> MPQHDQLHRYLFENFAVRGELVTVSETLQQILENHDYPQPVKNVLAELLVATSLLTATLKFDGDITVQLQGDGPMNLAVINGNNNQQMRGVARVQGEIPENADLKTLVGNGYVVITITPSEGERYQGVVGLEGDTLAADLEDYFMRSEQLPTRLFIRTGDVDGKPAAGG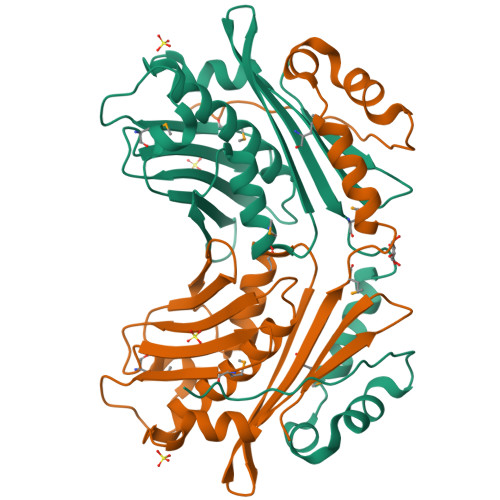MLLQVMPAQNAQQDDFDHLATLTETIKTEELLTLPANEVLWRLYHEEEVTVYDPQDVEFKCTCSRERSADALKTLPDEEVDSILAEDGEIDMHCDYCGNHYLFNAMDIAEIRNNASPADPQVH>[2x]MQGVRYIYHHFYTSLLVFVVMILFRSALSIYINTLSSTESLTISNNRTLVSPGDVFELGFFTPGSSSRWYLGIWYKKLSERTYVWVANRDNPLSNSTGTLKISGNNLVLRGDS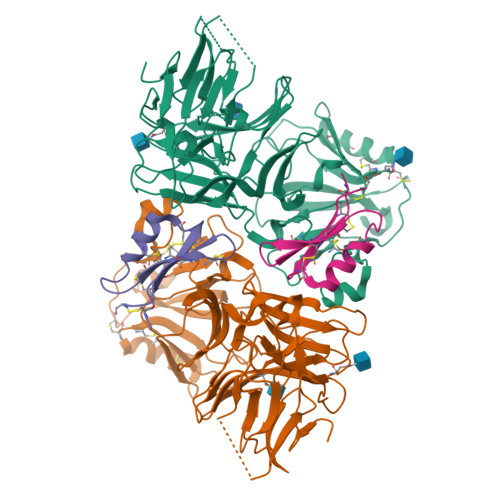NKSIWSTNLTRGNERSPVVAELLANGNFVMRDSNNNDASGFLWQSFDYPTDTLLPEMKLGYDLKTGRNRFLTSSRNSDDPSSGDYSYKLEPRRLPEFYLLQGDVREHRSGPWNGIQFSGIPEDQKSSYMVYNFTENSEEVAYTFRMTNNSFYSRLTINSEGYLERLTWAPSSGAWNVFWSSPNHQCDMYRMCGPYSYCDVNTSPSCNCIQGFNPGNVQQWALRNQISGCKRRTRLSCNGDGFTRMKNIKLPDTRMAIVDRSIGLKECEKRCLSDCNCTAFANADIRNRVTGCVIWTGELEDMRNYAEGGQDLYVRLAAADSRLEVLFQGP;>RCTRGFRKLGKCTTLEEEKCKTLYPRGQCTCSDSKMNTHSCDCKSC[2x]> GPGSMVSGSLVVAVDGPAGTGKSSVSRGLARALGARYLDTGAMYRIATLAVLRAGADLTDPAAIEKAAADAEIGVGSDPDVDAAFLAGEDVSSEIRGDAVTGAVSAVSAVPAVRTRLVDIQRKLATEGGRVVVEGRDIGTVVLPDADVKIFLTASAEERARRRNAQNVANGLPDDYATVLADV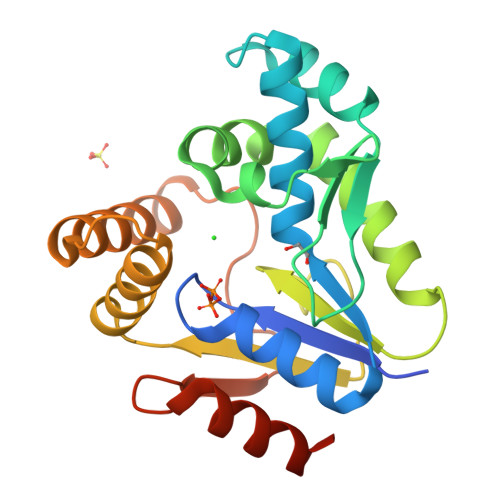QRRDHLDSTRPVSPLRAADDALVVDTSDMDQAQVIAHLLDLVTAQAGARR3-[3-(acetyloxymethyl)phenyl]benzoic 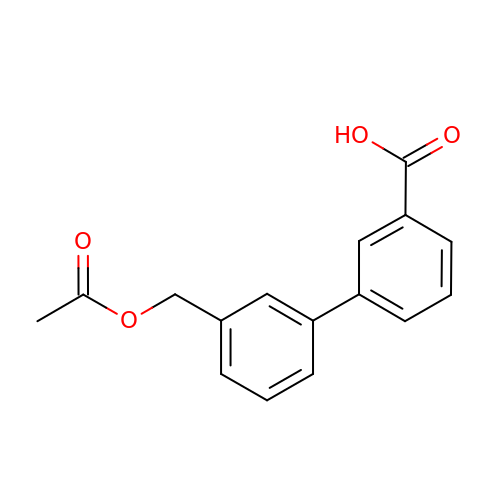acid | C16 H14 O4 | BHNLEDGKZQUQLL-UHFFFAOYSA-N>MSASHADQPTQTVSYPQLIDLLRRIFVVHGTSPEVADVLAENCASAQRDGSHSHGIFRIPGYLSSLASGWVDGKAVPVVEDVGAAFVRVDACNGFAQPALAAARSLLIDKARSAGVAILAIRGSHHFAALWPDVEPFAEQGLVALSMVNSMTCVVPHGARQPLFGTN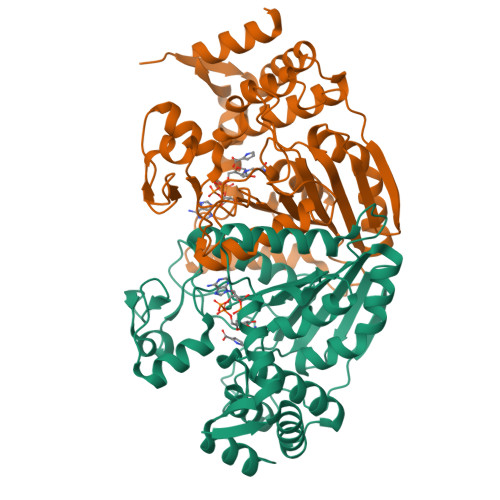PIAFGAPRAGGEPIVFDLATSAIAHGDVQIAAREGRLLPAGMGVDRDGLPTQEPRAILDGGALLPFGGHKGSALSMMVELLAAGLTGGNFSFEFDWSKHPGAQTPWTGQLLIVIDPDKGAGQHFAQRSEELVRQLHGVGQERLPGDRRYLERARSMAHGIVIAQADLERLQELAGH[2x]> 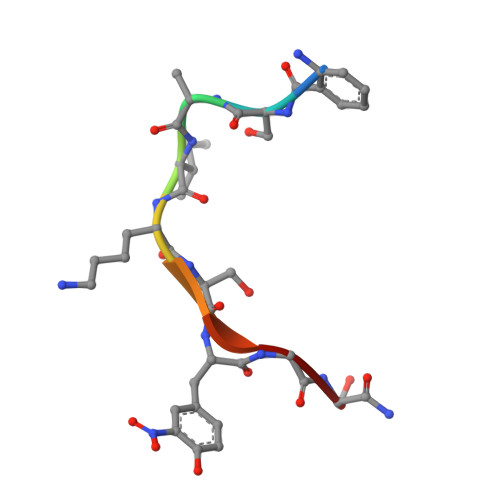XSAIKSYGS>CKGADGAHGVUGCPGTAGAAGSVGGPGCDGGHGGNGGNGNPGCAGGVGGAGGASGGTGVGGRGGKGGSGTPKGADGAPGAP[2x];>[2x]CKGADGAHGVNGCPGTAGAAGSV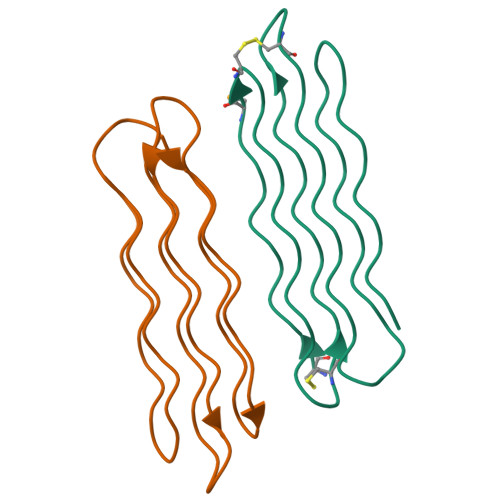GGPGCDGGHGGNGGNGNPGCAGGVGGAGGASGGTGVGGRGGKGGSGTPKGADGAPGAP4-azanyl-1~{H}-pyrazole-3,5-dicarboxylic 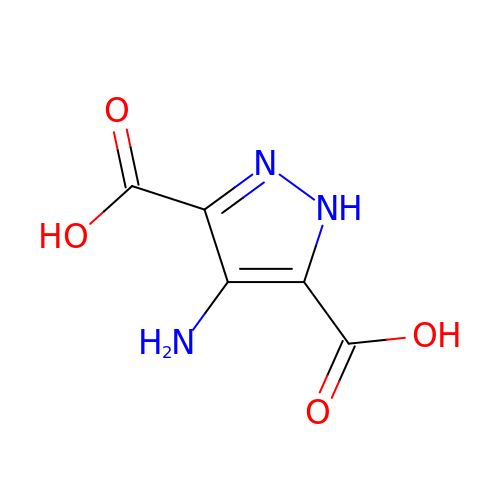acid | C5 H5 N3 O4 | IGUCGPRNZVGVNO-UHFFFAOYSA-N>KMAFTLADRVTEEMLADKAALVVEVVEENYHDAPIVGIAVVNEHGRFFLRPETALADPQFVAWLGDETKKKSMFDSKRAAVALKWKGIELCGVSFDLLLAAYLLDPAQGVDDVAAAAKMKQYEAVRPDEAVYGKGAKRAVPDEPVLAEHLVRKAAAIWELERPFLDELRRNEQDRLLVELEQPLSSILAEMEFAGVKVDTKRLEQMGKELAEQLGTVEQRIYELAGQEFNINSPKQLGVILFEKLQLPVLKKTKTGYSTSADVLEKLAPYHEIVENILHYRQLGKLQSTYIEGLLKVVRPATKKVHTIFNQALTQTGRLSSTEPNLQNIPIRLEEGRKIRQAFVPSESDWLIFAADYSQIELRVLAHIAEDDNLMEAFRRDLDIHTKTAMDIFQVSEDEVTPNMRRQAKAVNFGIVYGISDYGLAQNLNISRKEAAEFIERYFESFPGVKRYMENIVQEAKQKGYVTTLLHRRRYLPDITSRNFNVRSFAERMAMNTPIQGSAADIIKKAMIDLNARLKEERLQAHLLLQVHDELILEAPKEEMERLCRLVPEVMEQAVTLRVPLKVDYHYGSTWYDAK[2x]

Polymerases generate nascent strands of genetic material by stepwise phosphoryl transfer of nucleotides to primer termini, yielding O3′→P5′ phosphodiester linkages. We reported that 3′-NH2 primer extension can be catalyzed by a modified DNA polymerase, yielding N3′→P5′ phosphoramidate DNA (NP-DNA). The large fragment of DNA polymerase I (BF), cloned from the thermophilic soil bacterium Geobacillus stearothermophilus (Bst), acquires nontrivial levels of N3′→P5′ polymerase activity via two surprisingly minor substitutions: (A) a single active site mutation (F710Y) and (B) substitution of its divalent Mg2+ cofactors with Ca2+ (1). To add evidence that a single divalent metal ion cofactor catalyzes unnatural NP synthesis in BF, a polymerase A family member, we carried out a single nucleotide primer extension reaction in intact crystals.

Reactions were then initiated in the intact crystals by pH-shift from an acidic mother liquor (pH < 6) to a basic soaking liquor at pH 8.8, and reacting crystals were quenched at various times by flash freezing. Conformational changes in both the upstream and downstream nucleotides flanking the nascent bond are linearly correlated with covalent bonding. The downstream conformational change in the dGTP substrate sugar from C2′- to C3′-endo upon product formation, however, was not observed in an equivalent time-resolved experiment with the wild-type enzyme, in which the conformation is stably C3′-endo. Unlike for native phosphodiester catalysis, only a single metal ion cofactor is detectable by crystallography during NP catalysis. The lack of electron density for an A-site metal ion in the ground state and at later time points is also consistent with the expectation of a neutral nucleophile in the NP reaction and the generally weak affinity of aliphatic amines for Ca2+.>MLSFLLTLKRMLRACLRAWKDKEFQVLFVLTILTLISGTIFYSTVEGLRPIDALYFSVVTLTTVGAGNFEPQTDFGKIFTILYIFIGIGLVFGFIHKLAVNVQLPS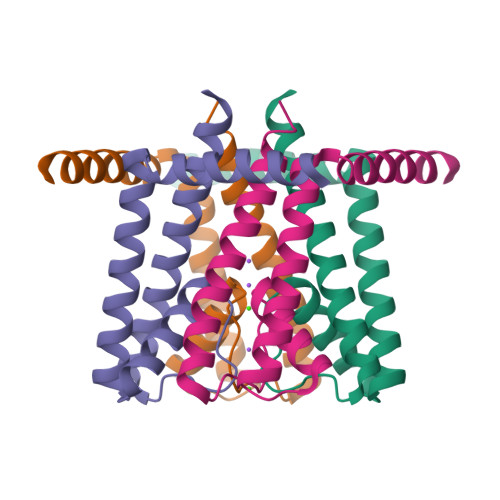ILSNLVPR[2x]MRG family proteins contain a chromodomain at the N-terminal and an MRG domain at the C-terminal end. As a “Royal Family” member, the N-terminal chromodomain functions as a histone reader that specifically recognizes methylated histone markers. MRG2 and MRG702 have been reported to be involved in floral transition, a highly regulated process in plant development between the vegetative stage and reproductive stage. Herein, we study the binding specificities of the chromodomains of MRG701 (the homologue of MRG702 in rice) and MRG1 (the homologue of MRG2 in Arabidopsis). Both the MRG701 chromodomain (MRG701CD) and the MRG1 chromodomain (MRG1CD) specifically bind to H3K36me3 and H3K4me3.

Only MRG701CD in complex with H3K36me3 produced crystals that diffracted to 1.4-Å. There are two MRG701CD molecules (molA and molB) in one asymmetric unit (AU), and the r.m.s.d. between these two molecules is 0.140 Å. The structure of MRG701CD adopts a compact fold with four β-strands shaped like a β-barrel and a C-terminal α-helix. The trimethylated lysine binding pocket was formed by the following five aromatic residues: H37, Y42, Y62, W65, and W69. However, no extra electron density was observed in the trimethylated lysine binding pocket. Comparing the structure with other MRG chromodomain structures, we found that W65 in the aromatic cage was stretched toward the center of the cage. The indole ring of W65 occupied the binding site of the trimethyl group in the lysine side chain. Two MRG701CD molecules are related via pseudo-2-fold symmetry in the crystal structure, and they form a dimer interface along the β2-strand of each molecule in an anti-parallel manner. Specifically, both E50 and K52 on β2 of molA form both hydrogen bonding and electrostatic interactions with K52’ and E50’ on β2’ of molB, respectively. In addition, W56 on β3 of molA contacts W56’ on β3’ of molB via π-π stacking interaction.

>GSFKEGERVLAYHGPLLYEAKVQKSENKEDEWRYHVHYLGWSKSWDEWVTNDRLLKLTDENIRKQQELEKSQ[2x]>[2x]DDLPYRFGLGKADITGEAAEVGMMGYSSLEQKTAGIHMRQWARAFVIEEAASGRRLVYVNTDLGMIFQAVHLKVLARLKAKYPGVYDENNVMLA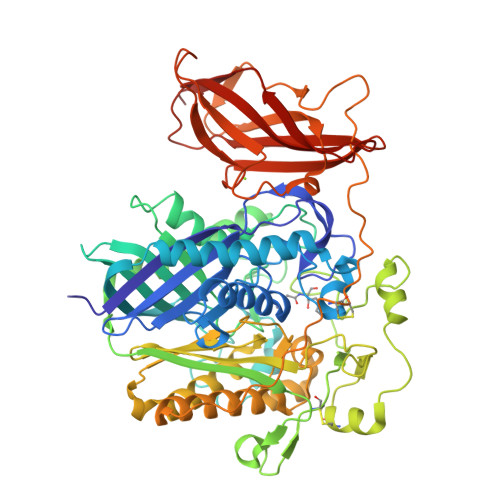ATHTHSGPGGFSHYAMYNLSVLGFQEKTFNAIVDGIVRSIERAQARLQPGRLFYGSGELRNASRNRSLLSHLKNPDIAGYEDGIDPQMSVLSFVDANGELAGAISWFPVHSTSMTNANHLISPDNKGYASYHWEHDVSRKSGFVAAFAQTNAGNLSPNLNLKPGSGPFDNEFDNTREIGLRQFAKAYEIAGQAQEEVLGELDSRFRFVDFTRLPIRPEFTDGQPRQLCTAAIGTSLAAGSTEDGPGPLGLEEGNNPFLSALGGLLTGVPPQELVQCQAEKTILADTGNKKPYPWTPTVLPIQMFRIGQLELLGAPAEFTVMAGVRIRRAVQAASEAAGIRHVVFNGYANAYASYVTTREEYAAQEYEGGSTLYGPWTQAAYQQLFVDMAVALRERLPVETSAIAPDLSCCQMNFQTGVVADDPYIGKSFGDVLQQPRESYRIGDKVTVAFVTGHPKNDLRTEKTFLEVVNIGKDGKQTPVTVATDNDWDTQYRWERVGISASKATISWSIPPGTEPGHYYIRHYGNAKNFWTQKISEIGGSTRSFEVLGTTP>SMHFVQQKVKVFRAADPLVGVFLWGVAHSINELSQVPPPVMLLPDDFKASSKIKVNNHLFHRENLPSHFKFKEYCPQVFRNLRDRFGIDDQDYLVSLTRNPPSESEGSDGRFLISYDRTLVIKEVSSEDIADMHSNLSNYHQYIVKCHGNTLLPQFLGMYRVSVDNEDSYMLVMRNMFSHRLPVHRKYDLKGSLVSREASDKEKVKELPTLRDMDFLNKNQKVYIGEEEKKIFLEKLKRDVEFLVQLKIMDYSLLLGIHDIIRGSEPEEEAPVREDESEVDGDCSLTGPPALVGSYGTSPEGIGGYIHSHRPLGPGEFESFIDVYAIRSAEGAPQKEVYFMGLIDILTQYDAKKKAAHAAKTVKHGAGAEISTVHPEQY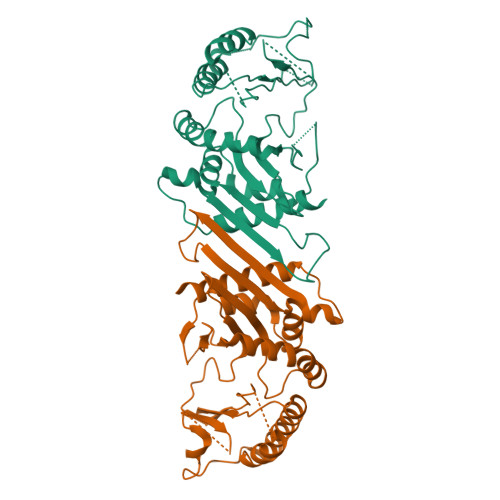AKRFLDFITNIFA[4x]N-{3-[(3R)-1-amino-3-methyl-3,4-dihydropyrrolo[1,2-a]pyrazin-3-yl]-4-fluorophenyl}-5-cyanopyridine-2-carboxamide 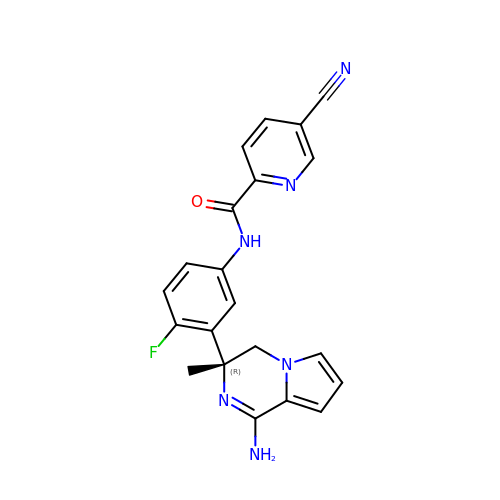| C21 H17 F N6 O | FZFJUKOAGOAQFB-NRFANRHFSA-N>KEVVLLDFAAAGGELGWLTHPYGKGWDLMQNIMNDMPIYMYSVCNVMSGDQDNWLRTNWVYRGEAERIFIELKFTVRDCNSFPGGASSCKETFNLYYAESDLDYGTNFQKRLFTKIDTIAPDEITVSSDFEARHVKLNVEERSVGPLTRKGFYLAFQDIGACVALLSVRVYYKKCPELLQGLAHFPETIAGSDAPSLATVAGTCVDHAVVPPGGEEPRMHCAVDGEWLVPIGQCLCQAGYEKVEDACQACSPGFFKFEASESPCLECPEHTLPSPEGATSCECEEGFFRAPQDPASMPCTRPPSAPHYLTAVGMGAKVELRWTPPQDSGGREDIVYSVTCEQCWPESGECGPCEASVRYSEPPHGLTRTSVT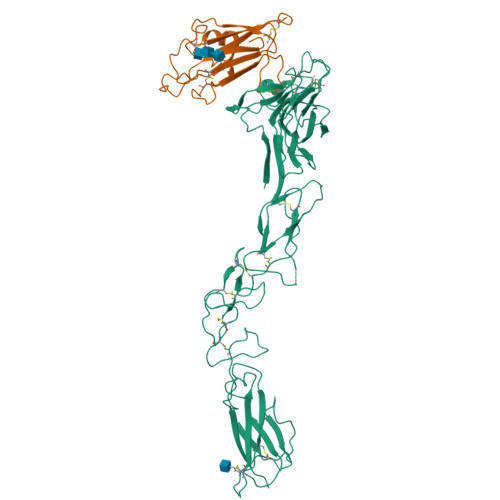VSDLEPHMNYTFTVEARNGVSGLVTSRSFRTASVSIN[2x];>VADRYAVYWNSSNPRFQRGDYHIDVCINDYLDVFCPHYEDSVPEDKTERYVLYMVNFDGYSACDHTSKGFKRWECNRPHSPNGPLKFSEKFQLFTPFSLGFEFRPGREYFYISSAIPDNGRRSCLKLKVFVRPTNSCM[2x]> CTSIVAQDSQGRIYHGRNLDYPFGKILRKLTADVQ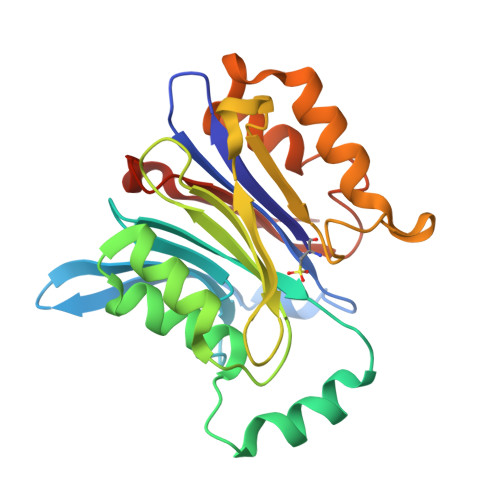FIKNGQIAFTGTTFVGYVGLWTGQSPHKFTISGDERDKGWWWENMIAALSLGHSPISWLIRKTLSESESFEAAVYTLAKTPLIADVYYIVGGTSPKEGVVITRDRGGPADIWPLDPLNGEWFRVETNYDHWKPAPKVDDRRTPAIKALNATGQAHLNLETLFQVLSLFPVYNSYTIYTTVMSAAEPDKYLTMIRNPS4,6-dimethylpyridin-2-amine | C7 H10 N2 | 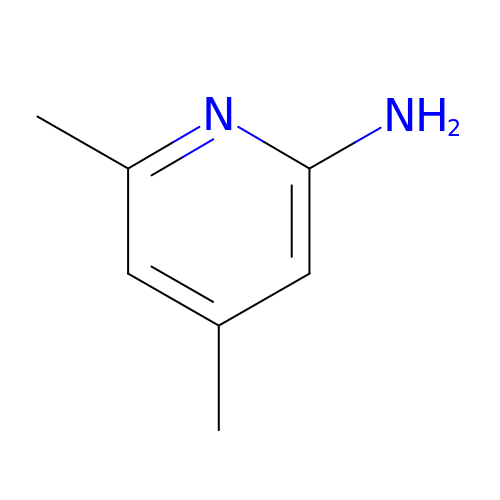BRBUBVKGJRPRRD-UHFFFAOYSA-N>[2x]MVSVSEIRKAQRAEGPATILAIGTANPANCVEQSTYPDFYFKITNSEHKTELKEKFQRMCDKSMIKRRYMYLTEEILKENPNVCEYMAPSLDARQDMVVVEVPRLGKEAAVKAIKEWGQPKSKITHLIVCTTSGVDMPGADYQLTKLLGLRPYVKRYMMYQQGSFAGGTVLRLAKDLAENNKGARVLVVCS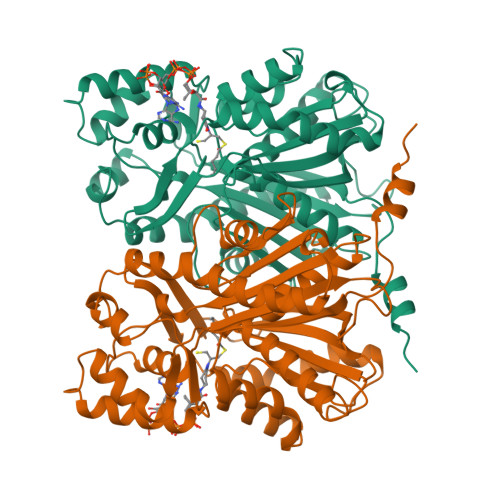EVTAVTFRGPSDTHLDSLVGQALFGDGAAALIVGSDPVPEIEKPIFEMVWTAQTIAPDSEGAIDGHLREAGLTFHLLKDVPGIVSKNITKALVEAFEPLGISDYNSIFWIAHPGGPAILDQVEQKLALKPEKMNATREVLSEYGNMSSACVLFILDEMRKKSTQNGLKTTGEGLEWGVLFGFGPGLTIETVVLRSVAI>RSPWTYCQVSQTLSLEDDPGRTFNWTSKAEQCNPGELCQETVLLIKADGTRTVVLASKSCVSQGGEAVTFIQYTAPPGLVAISYSNYCNDSLCNNKDSLASVWRVPETTATSNMSGTRHCPTCVALGS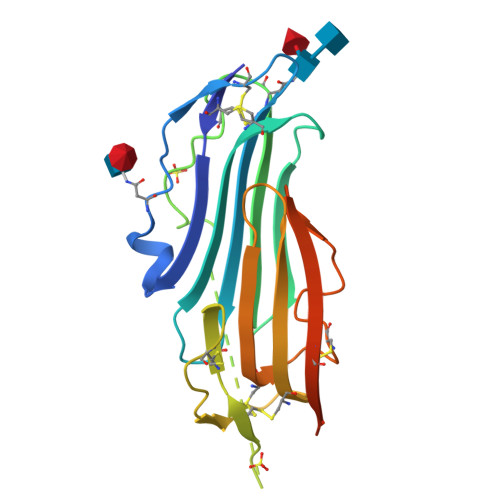CSSAPSMPCANGTTQCYQGRLEFSGGGMDATVQVKGCTTTIGCRLMAMIDSVGPMTVKETCSYQSFLQPRKAEIGEFLEVLFQ[2x]> SGNFCPLCDKCYDDDDYESKMMQCGKCDRWVHSKCENLSDEMYEILSNLPESVAYTCVNCTERHPAEWRLALEKELQISLKQVLTALLNSRTTSHLLRYRQQQPLDLEGVKRK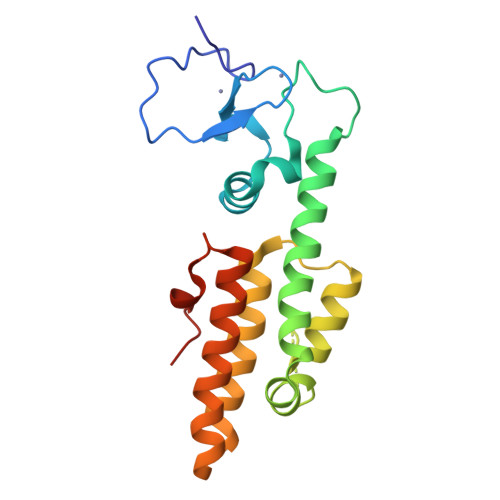MDQGNYTSVLEFSDDIVKIIQAAINSDGGQPEIKKANSMVKSFFIRQMERVFPWFSVKKSRFWEPNKVSS>[5x]MTKQHAFTREDLLR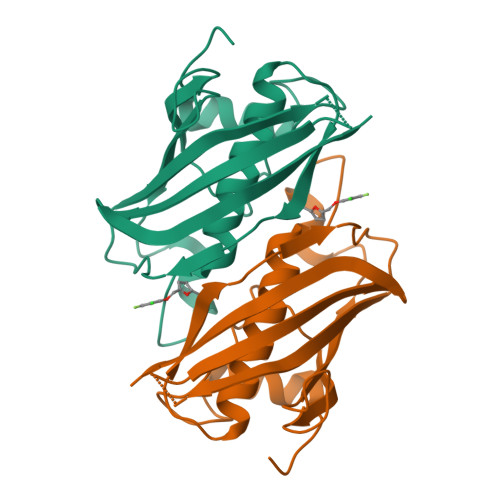CSRGELFGPGNAQLPAPNMLMIDRIVHISDVGGKYGKGELVAELDINPDLWFFACHFEGDPVMPGCLGLDAMWQLVGFYLGWQGNPGRGRALGSGEVKFFGQVLPTAKKVTYNIHIKRTINRSLVLAIADGTVSVDGREIYSAEGLRVGLFTSTDSF Kinetochores couple chromosomes to the mitotic spindle to segregate the genome during cell division. Knl1c functions in the spindle-assembly checkpoint (SAC), whereas Ndc80c, a heterotetramer of Ndc80, Nuf2, Spc24 and Spc25, is the major microtubule-binding component of KMN. Many fungi, including S. cerevisiae, utilize the ten-subunit Dam1 complex (Dam1c), which self-assembles into a large ring around microtubules, whereas most metazoans contain the Ska complex. Here we describe the cryo-electron microscopy structure of the budding yeast outer kinetochore Ndc80 and Dam1 ring complexes assembled onto microtubules.

The intermediate resolution of the cryo-EM map and the incompatible symmetries between the 16 protomers of the Dam1cRing and the 13 protofilament microtubule necessitated a divide and consolidate strategy for structure determination. This approach generated reconstructions of Ndc80c, and a dimer of Dam1c protomers at resolutions of 3.5 Å and 3.15 Å, respectively. Dam1cRing assembly follows a shoulder-to-shoulder configuration. Additionally, we resolved a ‘staple’ density located at the inter-Dam1cProtomer interfaces that was truncated from C. thermophilum Dam1 (38). The Dam1Staple comprises the N-terminus (residues 1-26) of the Dam1 subunit. The staple bridges the Dam1 and Dad1 subunits of Dam1cProtomerA with the Ask1 and Dad4 subunits of Dam1cProtomerB. Contact with Dam1cProtomerA is through hydrogen bonding between Dam1Staple residues Thr15 and Ser20, and Dad1A. Binding to Dam1cProtomerB is mediated by a salt bridge between Arg22 of Dad4B and Glu16 of Dam1Staple, as well as packing of Dam1Staple residues Tyr17, Leu19, and Ile21 against Ask1B and Dad4B. Serine 20 of Dam1Staple, a target of Aurora B kinase, is buried at the interprotomer interface close to Leu39, Asn40 and Asn43 of the Dad1 subunit of Dam1cProtomerA. Phosphorylation of Ser20 would cause steric hindrance and charge repulsion that would disrupt Dam1Staple binding. Our structure is consistent with previous cross-linking mass spectrometry and insertion mutagenesis experiments indicating that the central segment of the Ndc80:Nuf2 coiled-coils proximal to the conserved Ndc80 loop directly interacts with the Spc34:Spc19 C-termini.

>[2x]MQSSTSTDQHVLHHMDPHRFTSQIPTATSSQLRRRNSTNQGLTDMINKSIARNTISGTGIPTGGINKNKRTRSTVAGGTNGTALALNDKSNSRNSVSRLSINQLGSLQQHLSNRDPRPLRDKNFQSAIQEEIYDYLKKNKFDIETNHPISIKFLKQPTQKGFIIIFKWLYLRLDPGYGFTKSIENEIYQILKNLRYPFLESINKSQISAVGGSNWHKFLGMLHWMVRTNIKLDMCLNKVDRSLINQNTQEITILSQPLKTLDEQDQRQERYELMVEKLLIDYFTESYKSFLKLEDNYEPSMQELKLGFEKFVHIINTDIANLQTQNDNLYEKYQEVMKISQKIKTTREKWKALKSDSNKYENYVNAMKQKSQEWPGKLEKMKSECELKEEEIKALQSNISELHKILRKKGISTEQFELQNQEREKLTRELDKINIQSDKLTSSIKSRKLEAEGIFKSLLDTLRQYDSSIQNLTRSRSQLGHNVNDSSLKINISENLLDRDFHEGISYEQLFPKGSGINESIKKSILKLNDEIQERIKTIEKDNITLEKDIKNLKHDINEKTQINEKLELELSEANSKFELSKQENERLLVAQRIEIEKMEKKINDSNLLMKTKISDAEELVTSTELKLEELKVDLNRKRYKLHQQVIHVIDITSKFKINIQSSLENSENELGNVIEELRNLEFETEHNVTN;>MSRNQDVFPILDLQELVICLQSCDFALATQENISRPTSDYMVTLYKQIIENFMGISVESLLNSSNQETGDGHLQEENENIYLDTLNVLVLNKICFKFFENIGVQDFNMTDLYKPEAQRTQRLLSAVVNYARFREERMFDCNSFILQMESLLGQLRSKFDDYNLIQQQLKQYEDVDGDNIPDEQELQKLEEQNKELEIQLKKLTKIQETLSIDYNDYKISKQSIFKDLEALSFQIVELESNRDKLIKISNTDMEELSEGIKELNDLLIQRKKTLDDLTAQQKNLQDTVTTFETIISELYDVLRIISSEVQESNRTETELVGLKQNLINNKLKLMNVLETGIMYKLEILQEQLDLQLKNLEKLSQDTKEESRLNDTKLMDLQIKYENEIKPKIDKTDIFIQEELISGKINKLNDEIKQLQKDFEVEVKEIEIEYSLLSGHINKYMNEMLEYMQ[2x];>[3x]MSEDKAKLGTTRSATEYRLSIGSAPTSRRSSMGESSSLMKFADQEGLTSSVGEYNENTIQQLLLPKIRELSDSIITLDSNFTRLNFIHESLADLNESLGSLLYGIMSNSWCVEFSQAPHDIQDDLIAIKQLKSLEDEKNNLVMELSNMERGIKRKKDEQGENDLAKASQNKQFNQPLFPSSQVRKYRSYDNRDKRKPSKIGNNLQVENEEDYEDDTSSEASFVLNPTNIGMSKSSQGHVTKTTRLNNNTNSKLRRKSILHTIRNSIASGADLPIENDNVVNLGDLHPNNRISLGSGAARVVNGPVTKNRNSMFSGRAERKPTESRHSVAKKTEKKINTRPPFR;>[2x]MSEQSQLDDSTIDKLIPQIFNEMRSNLNNTTNKFPKSTGGGASDNISANSNSIRSFNSITTQSLLKESESLDKITAMIKNVTAALKNNLPVYVNQVHEVCKSTNSILDSWINIHSQAGYIHKLMSDQTYLKLINDRLHNENVNTNDEDGSTLHNVIALKKKEILDLRQKLENRKGEKDAAPAKPPNQGLNPRYGVQSGRRPVPSAGISNNGRVRKTHVPASKRPSGIPRVTNRWTKPTASSSRKMFR;>[2x]MDSIDEQIAIKRKELQSLQKITSLTDGLKIQLTELNEQIKEMGMNADSVAQLMNNWDSIINNISQASLGLLQYAEGDYEIGPWKDSKKKESEQSNETGLEAQENDKNDEDNDEDEDLVPLPETMVRIRVDGNE;>MMASTSNDEEKLISTTDKYFIEQRNIVLQEINETMNSILNGLNGLNISLESSIAVGREFQSVSDLWKTLYDGLESLSDEAPIDEQPTLSQSKTK[2x];>[2x]MENPHEQVQANILSRIIGNVKRLNESVAILNQELVTINNRNKNLEIMGAICDNYHSSVQFNLEATNNKKPPL;>[2x]MEHNLSPLQQEVLDKYKQLSLDLKALDETIKELNYSQHRQQHSQQETVSPDEILQEMRDIEVKIGLVGTLLKGSVYSLILQRKQEQESLGSNSK;>[2x]MGESLDRCIDDINRAVDSMSTLYFKPPGIFHNAILQGASNKASIRKDITRLIKDCNHDEAYLLFKVNPEKQSVSRRDGKEGVFDYVIKRDTDMKRNRRLGRPGEKPIIHVPKEVYLNKDRLDLNNKRRRTATTSGGGLNGFIFDTDLIGSSVISNSSSGTFKALSAVFKDDPQIQRLLYALENGSVLMEEESNNQRRKTIFVEDFPTDLILKVMAEVTDLWPLTEFKQDYDQLYHNYEQLSSKLRFIKKEVLLQDDRLKTMSQYHPSSSHDVAKIIRKEKDEIRRLEMEIANLQE;>MDSASKEETLEKLDQEITVNLQKIDSNLSFCFHKITQDIIPHVATYSEICERIMDSTEWLGTMFQETGLVNLQANAAAPVGNAPVKSLVSNNVGIFPTSAEEASRQSQTDNGPNEADSAVHVNRDVHSMFNNDSIDDFHTANITSTGQILKLPDSSDEDTGSEAVPSREQTDLTGEGHGGADDEQDESTIQRQSRKRKISLLLQQQYGSSSSMVPSPIVPNKMRKQLAHEEHINNDGDNDDENSNNIESSPLKQGHHHPKGQADDNNEGPDEEESTKEVPKPGTIIHFSTNR[2x];>MNANKQRQYNQLAHELRELQTNLQETTKQLDIMSKQCNENLVGQLGKVHGSWLIGSYIYYMEQMLGKTQ[2x];>MTDALEQSVLALEGTVSVLKDSVESLKCANEPSTNLASTMLQTKRVFRLVPEYDVERSKLDLIEEVEPLVRTLGDKLRKSMGRMQRELDTLQQTYELNDLRLKKNISMDDDDALNSPDMGQEYEGRDADDVVMMASSTNEELEELKKLKEKKKQLENKLEILKQK[2x]>GPLGSPEFQRTKPFSVPNIPMNLMSNSRVPMLIDGMMVSNDQNQVPQFQNGRVTLDGQLQGTTTVSAACIARMRGRIFNNNGNYGVNLAELDGNPYHAFDSPAPLGFPDFG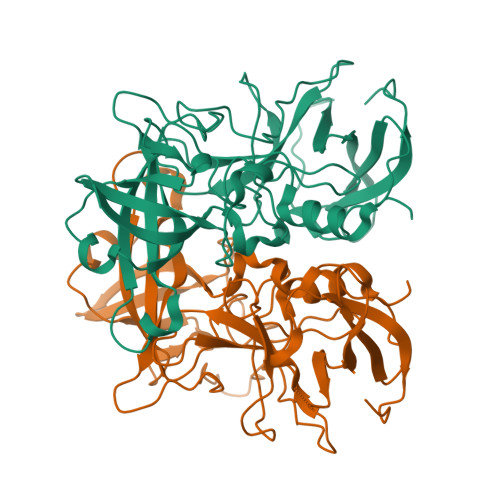NCDLHMTFVKINPTELSTGDPSGKVVIHSYDATFAPHLGTVKLEDNNELDQFVGKEVVLELTWVSNRTGATLNLWAVPNYGSNLTQASQLAPPIYPPGFGEAIVYFTSTFPTVSNPKVPCTLPQEFVSHFVNEQAPTRGDAALLHYVDPDTHRNLGEFKMYPEGYMTCVPNAGGGPQTLPINGVFVFISWVSRYYQL[2x]>GADDVVDSSKSFVMENFSSYHGTKPGYVDSIQKGIQKPKSGTQGNYDDDWKGFYSTDNKYDAAGYSVDNENPLSGK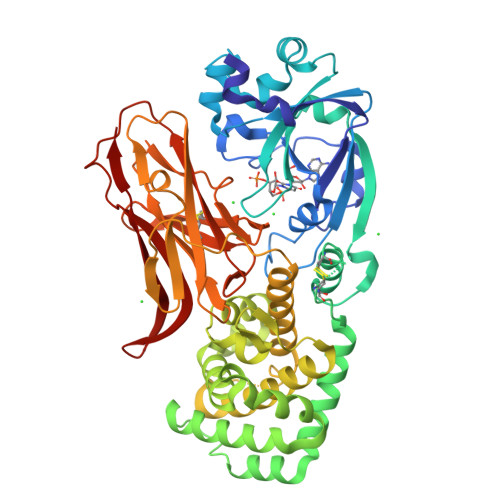AGGVVKVTYPGLTKVLALKVDNAETIKKELGLSLTEPLMEQVGTEEFIKRFGDGASRVVLSLPFAEGSSSVEYINNWEQAKALSVELEINFETRGKRGQDAMYEYMAQACAGNRVRRSVGSSLSCINLDWDVIRDKTKTKIESLKEHGPIKNKMSESPNKTVSEEKAKQYLEEFHQTALEHPELSELKTVTGTNPVFAGANYAAWAVNVAQVIDSETADNLEKTTAALSILPGIGSVMGIADGAVHHNTEEIVAQSIALSSLMVAQAIPLVGELVDIGFAAYNFVESIINLFQVVHNSYNRPAYSPGHKTQPFLHDGYAVSWNTVEDSIIRTGFQGESGHDIKITAENTPLPIAGVLLPTIPGKLDVNKSKTHISVNGRKIRMRCRAIDGDVTFCRPKSPVYVGNGVHANLHVAFHRSSSEKIHSNEISSDSIGVLGYQKTVDHTKVNSKLSLFFEIKS[2x]>[4x]SPLAAYEVDDSTGYLTSDVGGPIQDQTSLKAGIRGPTLLEDFMFRQKIQHFDHERVPERAVHARGAGAHGTFTSYADWSNITAASFLNATGKQTPVFVRFSTVAGSRGSADTARDVHGFATRFYTDEGNFDIVGNNIPVFFIQDAIQFPDLI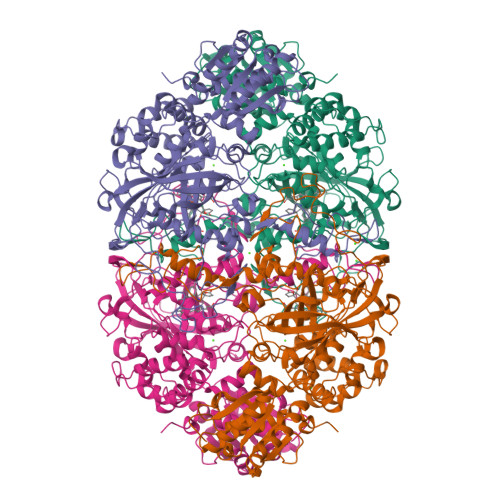HSVKPRPDNEIPQAATAHDSAWDFFSQQPSTMHTLFWAMSGHGIPRSYRHMDGFGVHTFRFVKDDGSSKLIKWHFKSRQGKASLVWEEAQVLSGKNADFHRQDLWDAIESGNGPEWDVCVQIVDESQAQAFGFDLLDPTKIIPFEYAPLTKLGLLKLDRNPTNYFAETEQVMFQPGHIVRGIDFTEDPLLQGRLFSYLDTQLNRNGGPNFEQLPINMPRVPIHNNNRDGAGQMFIHRNKYPYTPNTLNSGYPRQANQNAGRGFFTAPGRTASGALVREVSPTFNDHWSQPRLFFNSLTPVEQQFLVNAMRFEISLVKSEEVKKNVLTQLNRVSHDVAVRVAAAIGLGAPDADDTYYHNNKTAGVSIVGSGPLPTIKTLRVGILATTSESSALDQAAQLRTRLEKDGLVVTVVAETLREGVDQTYSTADATGFDGVVVVDGAAALFASTASSPLFPTGRPLQIFVDAYRWGKPVGVCGGKSSEVLDAADVPEDGDGVYSEESVDMFVEEFEKGLATFRFTDRFALDS> GSMEAIAKYDFKATADDELSFKRGDILKVLNEECDQNWYKAELNGKDGFIPKNYIEMKPHPWFFGKIPRAKAEEMLSKQRHDGAFLIRESESAPGDFSLSVKFGNDVQHFKVLRDGAGKYFLWVVKFNSLNEL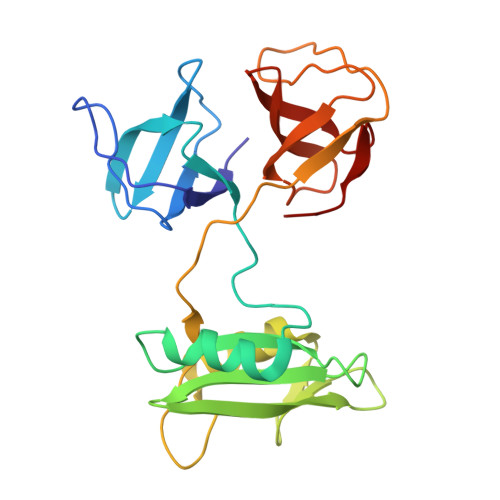VDYHRSTSVSRNQQIFLRDIEQVPQQPTYVQALFDFDPQEDGELGFRRGDFIHVMDNSDPNWWKGACHGQTGMFPRNYVTPVNRNV> MHHHHHHHHPDLGTGSENLYFQGAMADQVQDMYYLSPMQEGMLFHAILNPGQSFYLEQITMKVKGSLNIKCLEESMNVIMDRYDVFRTVFIHEKVKRPVQVVLKKRQFQIEEIDLTHLTGSEQTAKINEYKEQDKIRGFDLTRDIPMRAAIFKKAEESFEWVTSVHHIILDGWCIGIVVQDLFKVYNALREQKPYSLPPVKPYKDYIKWLEKQDKQASLRYWREYLEDFEGQTTFAEQRKKQKDGYEPKELLFSLPEAETKAFTELAKSQHTTLSTALQAVWSVLISRYQQSGDLAFGTVVSGRPAEIKGVEHMVGLFINVVPRRVKLSEGITFNDLLKQLQEQSLQSEPHQYVPLYDIQSQADQPKLIDHIIVFENYPLQDAKNEESSENGFDMVDVHVFEKSNYDLNLMASPGDEMLIKLAYNENVFDEAFILRLKSQLLTAIQQLIQNPDQPVSTINI

Nonribosomal peptides (NRPs) represent a valuable source of clinical therapeutics. These natural products are biosynthesized by multifunctional enzymatic assembly lines, called nonribosomal peptide synthetases (NRPSs), that use dedicated modules to incorporate each building block selectively and sequentially into the peptide scaffold. NRPS modules typically possess three core domains, which perform substrate selection and activation (adenylation or A domains), shuttling of activated substrates (thiolation or T domains, also called peptide carrier proteins, PCP or CP domains) and peptide bond formation (condensation or C domains), respectively. The enzymatic assembly line that produces the microbial lipopeptide antibiotic surfactin, surfactin synthetase, consists of the following three proteins: trimodular SrfA-A, trimodular SrfA-B and monomodular SrfA-C. The modules are composed of several functional domains, including C, A and T domains. In the current study, we re-engineered the donor substrate specificity of the SrfA-C C domain (green) to enable direct acylation of the acceptor Leu (residue 7, yellow highlight) with a fatty acid rather than an amino acid.

To gain insight into how the engineered SrfA-CFA variant recognizes and processes a lipid substrate, we attempted to crystallize its C domain in complex with substrate analogs. Two unrelated, highly diffracting crystal forms of the SrfA-CFA C domain were obtained and used to solve apo structures to high resolution. Variant 10, harboring mutations W143T, Y145V and F155I, was found to be the best catalyst for rapid fatty acylation of l-Leu, giving an apparent rate constant of 38 ± 7 min−1. In the SrfA-CFA structures, all mutations are clearly visible in electron density maps and introduce more space between the middle of helix 4 and the β sheet. Introduction of the W143T, Y145V and F155I mutations causes the following three connected changes: (1) the N-terminus of helix 4 shifts inward, toward the pocket mutations, by up to 2 Å; (2) the helix’s capping residue, Trp153, swings over to interact with the base of the latch; and (3) the latch shifts to pack Leu360 into the mutated pocket. However, in this conformation, the active site is not connected to the expanded mutated pocket, mainly because of the position of Glu37 and Leu360. Nevertheless, a reasonable 10-undecynoyl-ppant-TycA* model can be made that positions the distal end of the 10-undecynoyl moiety into the expanded pocket. Although this model is consistent with the mutations improving activity, cocrystal structures will ultimately be required to corroborate the proposed binding mode. Structure-based considerations would certainly have included mutation of Glu37 to a smaller residue, as the side chain of Glu37 blocks the fatty acid pocket in all crystal structures.> GCUCGGCGGUGGGGGAGCAUCUCCUGUAGGGGAGAUGUAACCCCCUUUACCUGCCGAACCCCGCCAGGCCCGGAAGGGAGCAACGGUAGGCAGG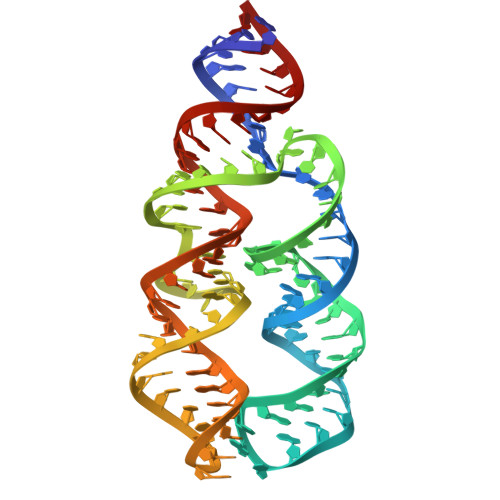ACGUCGG> MRGNIRVYCRIRPALKNLENSDTSLINVNEFDDNSGVQSMEVTKIQNTAQVHEFKFDKIFDQQDTNVDVFKEVGQLVQSSLDGYNVCIFAYGQTGSGKTFTMLNPGDGIIPSTISHIFNWINKLKTKGWDYKVNCEFIEIYNENIVDLLRSDNNNKEDTSIGLKHEIRH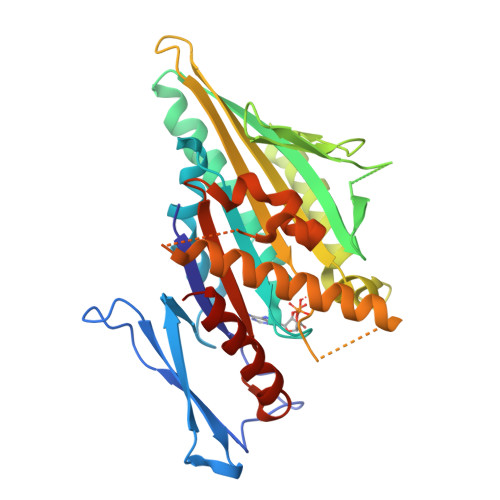DQETKTTTITNVTSCKLESEEMVEIILKKANKLRSTASTASNEHSSRSHSIFIIHLSGSNAKTGAHSYGTLNLVDLAGSERINVSQVVGDRLRETQNIKKSLSCLGDVIHALGQPDSTKRHIPFRNSKLTYLLQYSLTGDSKTLMFVNISPSSSHINETLNSLRFASKVNSTRLVSRK> GSQSRSIQTFPQPDTSVINGPDRPAGIPDPAGTTVAGGGAVYTVVPHLSMPHWAAQDFAKSLQSFRLGCANLKNRQGWQDVCAQAFQTPIHSFQAKRFFERYFTPWQVAGNGSLAGTVTGYYEPVLKGDGRRTERARFPIYGIPDD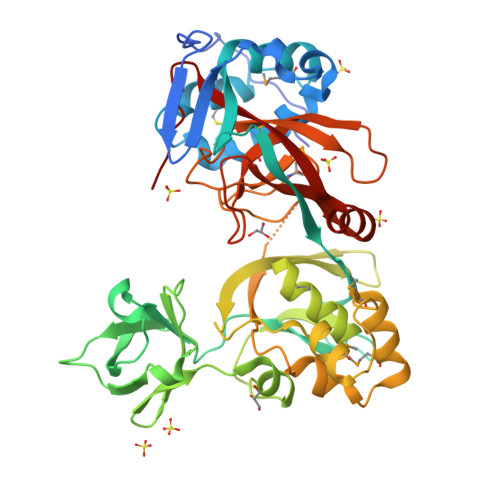FISVPLPAGLRGGKNLVRIRQTGKNSGTIDNAGGTHTADLSRFPITARTTAIKGRFEGSRFLPYHTRNQINGGALDGKAPILGYAEDPVELFFMHIQGSGRLKTPSGKYIRIGYADKNEHPYVSIGRYMADKGYLKLGQTSMQGIKAYMRQNPQRLAEVLGQNPSYIFFRELAGSGGDGPVGALGTPLMGEYAGAIDRHYITLGAPLFVATAHPVTRKALNRLIMAQDTGSAIKGAVRVDYFWGYGDEAGELAGKQKTTGYVWQLLPNGMKPEYRP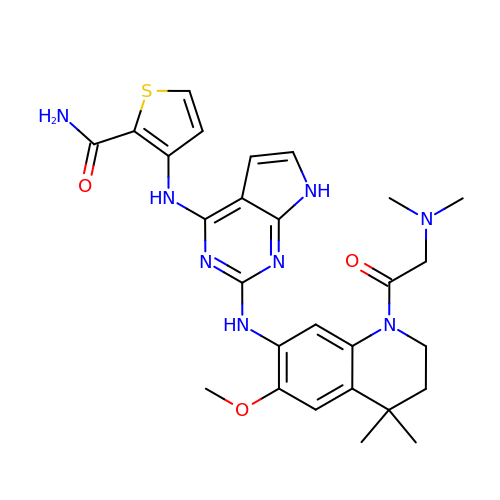3-[(2-{[1-(N,N-dimethylglycyl)-6-methoxy-4,4-dimethyl-1,2,3,4-tetrahydroquinolin-7-yl]amino}-7H-pyrrolo[2,3-d]pyrimidin-4-yl)amino]thiophene-2-carboxamide | C27 H32 N8 O3 S | YNSCKPCDFIDINW-UHFFFAOYSA-N>MAHHHHHHMIYAGVLQHAYCGSRKKTIEHTANLLEQALKKHPKTNLVVLQELNPYSYFCQSENPKFFDLGEYFEEDKAFFSALAQKFQVVLIASLFEKRAKGLYHNSAVVFEKDGSIAGVYRKMHIPDDPGFYEKFYFTPGDLGFEPIITSVGKLGLMVCWDQWYPEAARIMALKGAEILIYPSAIGFLE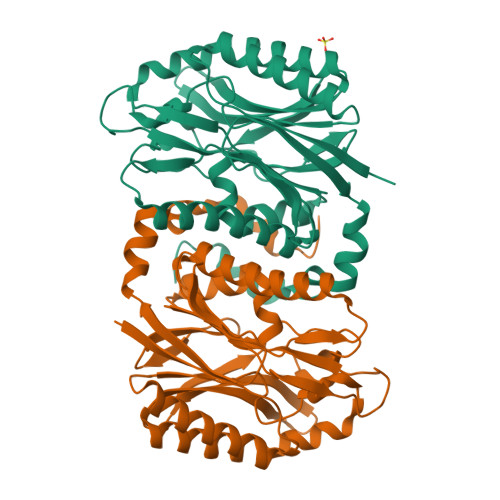EDSNEEKKRQQNAWETIQRGHAIANGLPLIATNRVGVELDPSGAIKGGITFFGSSFVVGALGEFLAKASDKEEILYAEIDLERTEEVRRMWPFLRDRRIDFYNDLLKRYI[4x]>LEIKRYKNRVASRKSRAKFKQLLQHYREVAAAKSSENDRLRLLLKQMCPSLDVD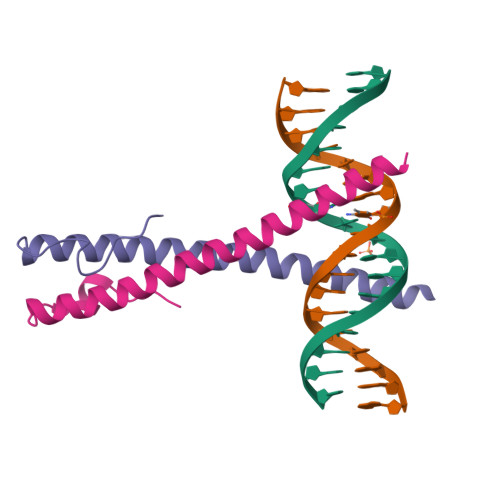SIIPRTPD[2x]>MEQAMRERSELARKGIARAKSVVALAYAGGVLFVAENPSRSLQKISELYDRVGFAAAGKFNEFDNLRRGGIQFADTRGYAYDRRDVTGRQLANVYAQTLGTIFTEQAKPYEVELCVAEVAHYGETKRPELYRITYDGSIADEPHFVVMGGTTEPIANALKESYAENASLTDALRIAVAALRAGSADTSGGDQPTLGVASLEVAVLDANRPRRAFRRITGSALQALLVDQESPQSDGESSG[14x];>TTIVALKYPGGVVMAGDRRSTQGNMISGRDVRKVYITDDYTATGIAGTAAVAVEFARLYAVELEHYEKLEGVPLTFAGKINRLAIMVRGNLAAAMQGLLALPLLAGYDI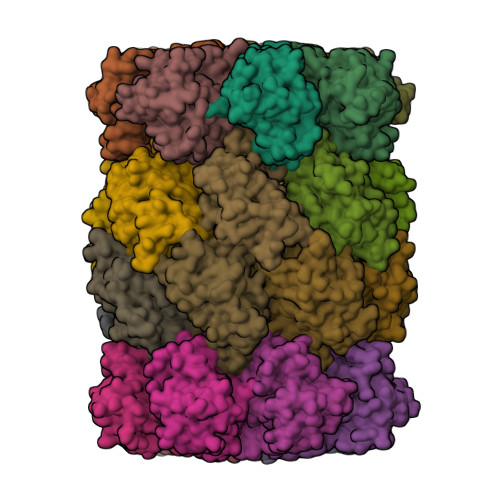HASDPQSAGRIVSFDAAGGWNIEEEGYQAVGSGSLFAKSSMKKLYSQVTDGDSGLRVAVEALYDAADDDSATGGPDLVRGIFPTAVIIDADGAVDVPESRIAELARAIIESRSGADTFGSDGGEK[14x]> VTSYTLSDVVS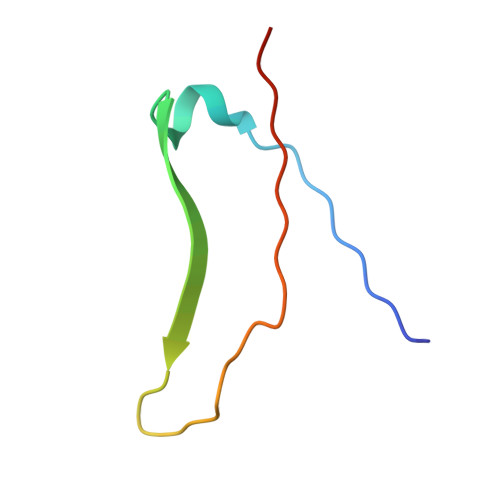LKDVVPEWVRIGFSATTGAEYAAHEVLSWSFHSELSGT> MEIPVIEPLFTKVTEDIPGAEGPVFDKNGDFYIVAPEVEVNGKPAGEILRIDLKTGKKTVICKPEVNGYGGIPAGCQCDRDANQLFVADMRLGLLVVQTDGTFEEIAKKDSEGRRMQGCNECAFDYEGNLWITAPAGEVAPADYTRSMQEKFGSIYCFTTDGQMIQVDTAFQFPNGIAVRHMNDGRPYQLIVAETPTKKLWSYDIKGPAKIENKKVWGHIPGTHEGGADGMDFDEDNNLLVANWGSSHIEVFGPDGGQPKMRIRCP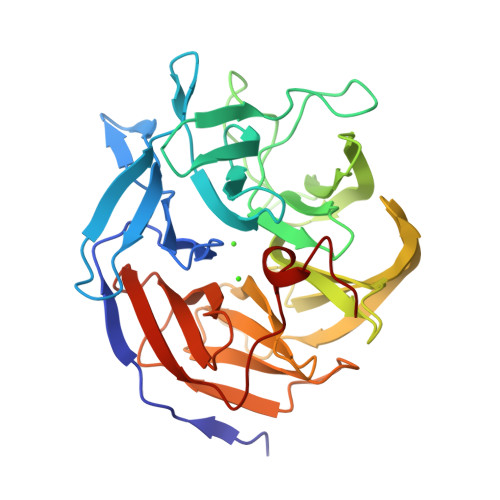FEKPSNLHFKPQTKTIFVTEHENNAVWKFEWQRNGKKQYCETLKFGIF> SERPFFCNFCGKT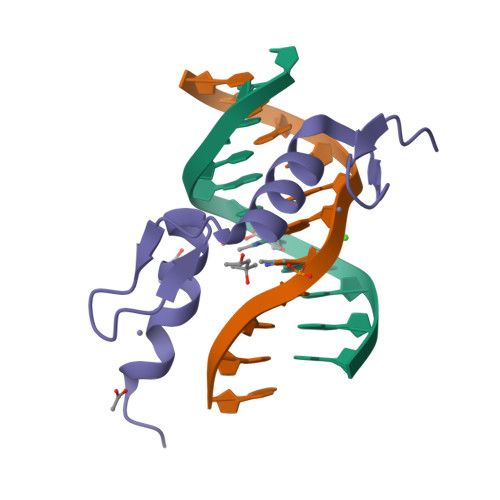YRDASGLSRHRRAHLGYRPRSCPECGKCFRDQSEVNRHLKVHQNKPA>VMKQYLSRLASLTLFVGFMSAAQAAVAPLDLVQPISDYKIYVSENLQTLVRDTREFTNAVKAGDVAKAKKLFA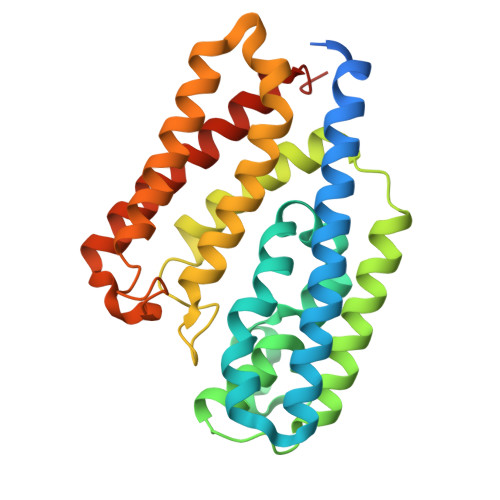STRMSYERIEPIAELFSDLDASIDSRADDHEKAEKDPAFFGFHRIEYGLFAQNSAKGLAPVADKLMADVLELQKRIRGLTFPPEKVVGGAAVLMEEVAATKISGEEDRYSHTDLWDFQANFEGAKKIVDLFRPLVVKDNRAFADKVDANFDTVFKTLAKYRTADGGFELYGKLSERDRKVLAGRVNTLAEDLSKMRGLLGLDLEHHHHHH[2x]>MGSDKIHHHHHHMKVKILVDSTADVPFSWMEKYDIDSIPLYVVWEDGRSEPDEREPEEIMNFYKRIREAGSVPKTSQPSVEDFKKRYLKYKEEDYDVVLVLTLSSKLSGTYNSAVLASKEVDIPVYVVDTLLASGAIPLPARVAREMLENGATIEEVLKKLDERMKNKDFKAIFYVSNFDYLVKGGRVSKFQGFVGNLLKIRVCLHIENGELIPYRKVRGDKKAIEALIEKLREDTPEGSKLRVIGVHADNEAGVVELLNTLRKSYEVVDEIISPMG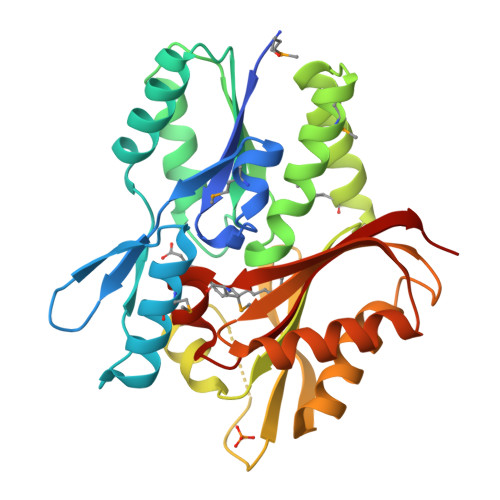KVITTHVGPGTVGFGIEVLERKR[2x]>[2x]MFEARLVQGSILKKVLEALKDLINEACWDISSSGVNLQSMDSSHVSLVQLTLRSEGFDTYRCDRNLAMGVNLTSMSKILKCAGNEDIITLRAEDNADTLALVFEAPNQEKVSDYEMKLMDLDVEQLGIPEQEYSCVVKMPSGEFARICRDLSHIGDAVVISCAKDGVKFSASGELGNGNIKLSQTSNVDKEEEAVTIEMNEPVQLTFALRYLNFFTKATPLSSTVTLSMSADVPLVVEYKIADMGHLKYYLAPK;> HMFEARLVQGSILKKVLEALKDLINEACWDISSSGVNLQSMDSSHVSLVQLTLRSEGFDTYRCDRNLAMGVNLTSMSKILKCAGNEDIITLRAEDNADTLALVFEAPNQEKVSDY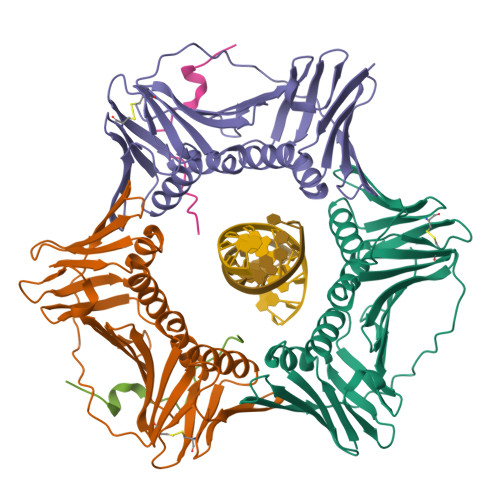EMKLMDLDVEQLGIPEQEYSCVVKMPSGEFARICRDLSHIGDAVVISCAKDGVKFSASGELGNGNIKLSQTSNVDKEEEAVTIEMNEPVQLTFALRYLNFFTKATPLSSTVTLSMSADVPLVVEYKIADMGHLKYYLAPKI;>PVCVRPTPKWQKGIGEFFRL[2x]PgDPP11 exhibits a strict substrate specificity for acidic residues (Asp/Glu) at the P1 position (NH2-P2-P1-P1’-P2’-…, where the P1-P1’ bond is the scissile bond), whereas PgDPP7 exhibits a broad substrate specificity for both aliphatic and aromatic residues at the P1 position. PgDPP11 is a homodimer, and each subunit contains a peptidase domain, including a double β-barrel fold that is characteristic of the chymotrypsin superfamily, as well as an unusual α-helical domain that regulates the exopeptidase activity of PgDPP11. Biochemical studies and crystal structure analyses revealed that Arg673 in the S1 subsite of PgDPP11 is a crucial residue for the strict Asp/Glu P1 specificity of PgDPP1123,27,31.

The crystal structure of PgDPP11 in complex with citrate and potassium ions was determined at a 1.50 Å resolution by analyzing a space-grown crystal. Two protomers of PgDPP11 are related by a crystallographic two-fold axis of the C2221 crystal and form a dimer. High-resolution diffraction data obtained from a space-grown crystal enabled us to identify two potassium ion-binding sites and two citrate ion-binding sites in the protomer of PgDPP11 because the present crystallization conditions contained 0.20 M tri-potassium citrate in the reservoir solution. In this study, the citrate ion was identified in the S1 subsite of PgDPP11, and the other was identified on the surface of the molecule and found to interact with the side chain of Arg536. A distal carboxy group (O3C5O4) of the citrate ion forms bifurcated salt bridges with the side chain of Arg673 (O4(citrate)–NE(Arg673): 2.8 Å and O3(citrate)–NH2(Arg673): 2.8 Å) and is found to mimic the binding mode of an acidic (Asp/Glu) side chain of the P1 residue of a substrate peptide. A water molecule that is hydrogen bonded to the central carboxy group (O5C6O6) of the citrate (O6(citrate)–O(HOH240): 2.9 Å) is accommodated in the oxyanion hole of PgDPP11 (N(Gly653)–O(HOH240): 2.9 Å and N(Ser655)–O(HOH240): 3.0 Å). In addition, a potassium ion was identified in the P2 residue-binding site of PgDPP11 and found to mimic the binding mode of the positively charged N-terminus of the P2 position of the substrate peptide. The other potassium ion was found at the bottom of the S1 subsite and appeared to be trapped by an electrostatic interaction with the side chain of Asp681. Comparison the binding mode of the citrate ion described above and a dipeptide docking model of PgDPP1127 indicates that the potassium ion, the carboxy group of citrate and the water molecule (HOH240) mimic the binding sites of the N-terminus, the acidic P1 side chain and the carbonyl group of the P1 residue of the bound peptide, respectively. The bound citrate ion, a potassium ion, and a water molecule in the S1 subsite of PgDPP11 were regarded to mimic the binding of an acidic amino acid and were utilized as a pharmacophore for an in silico inhibitor screening.

> MKKRLLLPLFAALCLSQIAHADEGMWLMQQLGRKYAQMKERGLKMKEYDLYNPNGTSLKDAVVLFDGGCTGEVVSDRGLVLTNHHCGYDMIQAHSTLEHNYLENGFWAMREADELPNKDISVVFIDKIEDVTDYVKKELKAIKDPNSMDYLSPKYLQKLADKKAGKNFSAKNPGLSVEIKAFYGGNLYLMFTKKTYTDVRLVGAPPSSIGKFGADTDNWIWPRHTGDFSIFRIYADKNGNPAPYSEDNVPLKPKRFFNISLGGVQENDYAMIMGFPGTTHRYFTASEVDEWKSIDNDIRIRMRDIRQGVMLREMLADPQIKIMYSAKYAASQNAYKRAIGANWAIKTRGLRQNKQAMQDRLIAWGAKQGTPRYEEAVHEIDATVAKRADLRRRYWMIEEGIIRGIEFARSPIPTEDETKALQGNDASARKEAIDKIRTRYSKFANKDYSAEVDKKVAVAMLTEYLKEIPYENLPLHLRLVKDRFAGDVQAYVDDIFARSVFGSEAQFDAFAAVPSVEKLAEDPMVLFASSVFDEYRKLYNELRPYDDPILRAQRTYIAGLLEMDGDQDQFPDANLTLRFTYGQVKGYSPRDNVYYGHQTTLDGVMEKEDPDNWEFVVDPKLKAVYERKDFGRYADRSGRMPVAFCATTHTTGGNSGSPVMNANGELIGLNFDRNWEGVGGDIQYLADYQRSIIVDIRYVLLVIDKVGGCQRLLDEMNIVP>[2x]HHHHHHENLYFQGKEWQENKSWNAHFTEHKSQGVVVLWNENKQQGFTNNLKRANQAFLPASTFKIPNSLIALDLGVVKDEHQVFKWDGQTRDIATWNRDHNLITAMKYSVVPVYQEFARQIGEARMSKMLH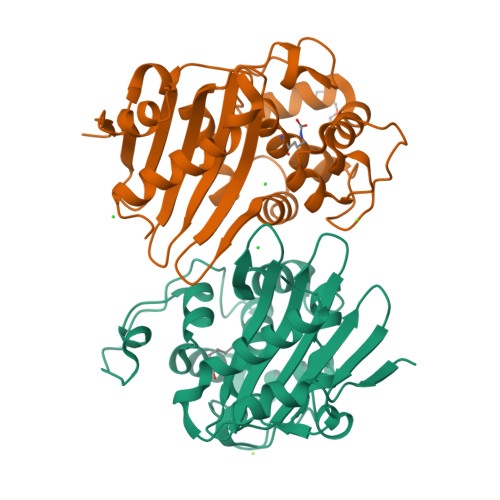AFDYGNEDISGNVDSFWLDGGIRISATEQISFLRKLYHNKLHVSERSQRIVKQAMLTEANGDYIIRAKTGYDTKIGWWVGWVELDDNVWFFAMNMDMPTSDGLGLRQAITKEVLKQEKIIP>MAKANSSFSEVQIARRIKEGRGQGHGKDYIPWLTVQEVPSSGRSHRIYSHKTGRVHHLLSDLEL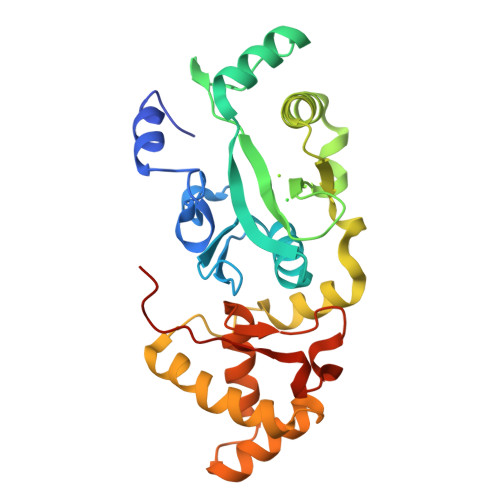AVFLSLEWESSVLDIREQFPLLPSDTRQIAIDSGIKHPVIRGVDQVMSTDFLVDCKDGPFEQFAIQVKPAAALQDERTLEKLELERRYWQQKQIPWFIFTDKEINPVVKENIEWLYSVKTEEVSAELLAQLSPLAHILQEKGDENIINVCKQVDIAYDLELGKTLSEIRALTANGFIKFNIYKSFRANKCADLCISQVVNMEELRYVAN[2x]6-NITROBENZOTRIAZOLE | C6 H4 N4 O2 | 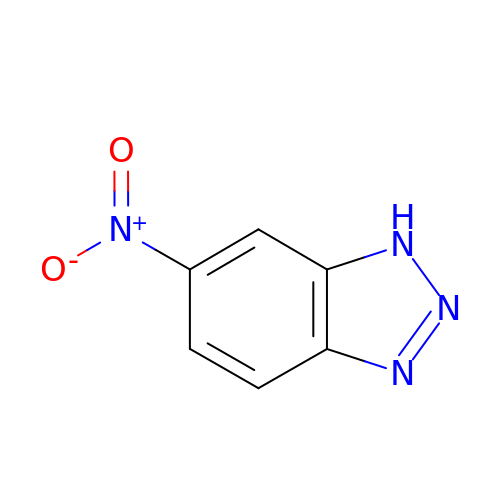AOCDQWRMYHJTMY-UHFFFAOYSA-N> MSTVTITDLARENVRNLTPYQSARRLGGNGDVWLNANEYPTAVEFQLTQQTLNRYPECQPKAVIENYAQYAGVKPEQVLVSRGADEGIELLIRAFCEPGKDAILYCPPTYGMYSVSAETIGVECRTVPTLDNWQLDLQGISDKLDGVKVVYVCSPNNPTGQLINPQDFRTLLELTRGKAIVVADEAYIEFCPQASLAGWLAEYPHLAILRTLSKAFALAGLRCGFTLANEEVINLLMKVIAPYPLSTPVADIAAQALSPQGIVAMRERVAQIIAEREYLIAALKEIPCVEQVFDSETNYILARFKASSAVFKSLWDQGII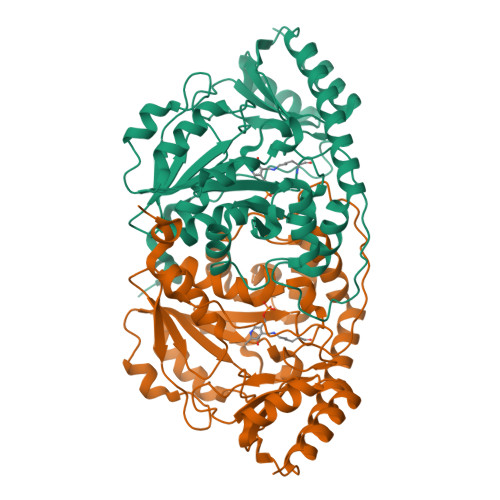LRDQNKQPSLSGCLRITVGTREESQRVIDALRAEQV The endonuclease domain is at the N-terminus of the L protein, a multifunctional protein that includes the RNA-dependent RNA polymerase. The synthesis of mRNA in arenaviruses is a process that is primed by capped nucleotides that are ‘stolen’ from the cellular mRNA by the endonuclease domain in cooperation with other domains of the L protein. The L protein cleaves and snatches the native cellular mRNA cap structure through its endonuclease domain after ∼11 nucleotides, and uses it as a primer sequence for the RdRp domain of the L protein to synthesize the viral mRNA. The catalytic centre of the ENDO resides in the N-terminal part around Asp88 and should contain two Mg2+ (or Mn2+) ions, which are critical for the RNA-cleavage mechanism.

The crystal structure of the LCMV endonuclease domain (ENDO) was originally determined some time ago, but in this original structure the catalytic ions necessary to fully understand the mode of action of the endonuclease were missing. Therefore, for this structural study to be successful it was critical to search for new crystallization conditions that would allow the molecules to form ionic complexes. The present ENDO-WT structure clearly shows the two Mg2+ ions directly coordinated by the catalytic Asp88 and, through a network of water molecules, by Glu101 and Lys114. From our observation of 100 crystals during the screening and analysis of work performed on the Lassa virus endonuclease domain, this coordination event seems to be rare. On the other hand, if we compare these results with the structure of the Lassa virus endonuclease domain reported by Reguera et al., we can see that the coordination of the two Mn2+ ions involved the corresponding residues Asp89, Glu102 and Lys115, a residue from the asymmetric unit (Glu3) and no waters. Together, these data indicate that the affinity of the Arenaviridae endonuclease for its catalytic ions is low and that the metal-ion binding at the catalytic site is the result of a random event in the absence of an RNA substrate. In the ENDO-WT structure, the water molecules mimic the positions of the nonbridged O atoms of the RNA phosphodiester backbone involved in binding to the ions. Therefore, we propose that in the case of the LCMV endonuclease domain the RNA substrate is a necessary contributor to the formation of a transitioning ion-binding/catalytic site that allows a two-metal-ion catalytic mechanism (TMIC). Our data show that the presence of ions in the holo structure is in fact a rare event. The structures show that the metal-ion binding depends on the number of water molecules that are able to create a mesh of interaction around the ions. This suggests that the catalytic ions responsible for the two-metal-ion catalysis reaction are most likely brought in by the RNA substrate itself.

>[2x]MKHHHHHHDEIISELRELCLNYIEQDERLSRQKLNFLGQREPRMVLIEGLKLLSRCIEIDSADKSGCTHNHDDKSVETILVESGIVCPGLPLIIPDGYKLIDNSLILLECFVRSTPASFEKKFIEDTNKLACIREDLAVAGVTLVPIVDGRCDYDNSFMPEWANFKFRDLLFKLLEYSNQDEKVFEESEYFRLCESLKTTIDKR BIS-(2-ACETAMIDO-2-DEOXY-ALPHA-D-GLUCOPYRANOSYLOXYCARBONYL)-4,7,10-TRIOXA-1,13-TRIDECANEDIAMINE | C28 H50 N4 O17 | 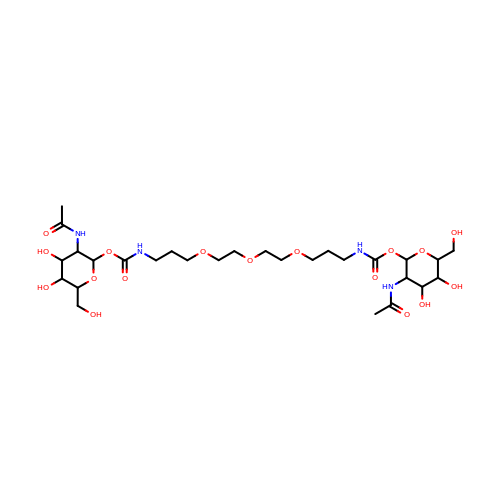RLNVSMVMMKEUND-VCVUPCPRSA-N>CCCCATGGG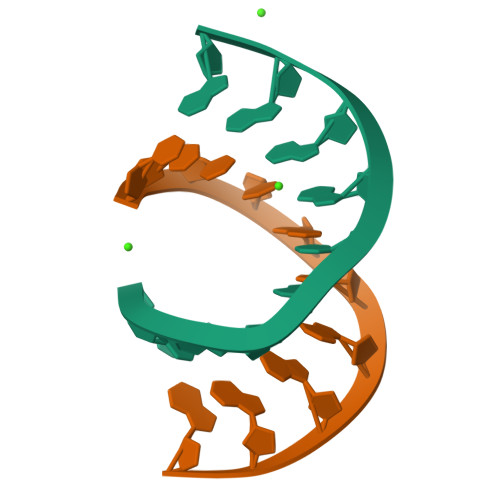G[2x]>[2x]MRPETIPGISLNEDNSHYFYTRAGRRLSAEEVDSWVDQYAGTQVKELMLCPNCMRTSYASQVWDPIWRGYDPAGPDDQPLLASLPPEERVAARGWIHTAWQLHQDGIDIYARWIRRCRQRGISPWISMRMNDVHYVNDERCFLHSEFWRENPQLRRVPYRFAEWTDRAFDYGRAEVREHH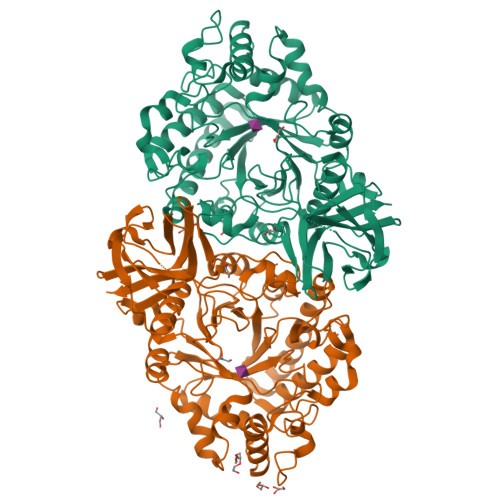LKLIRELAARYDFDGLELDWMRFGFHFRPGYEAEGAEILTAFTAEVRRLLDDWEKRRGHKIHLGARIPSRPATALGLGMDAVTWARRGLVDMLVITPFWASAETDMPVEIWRQLLEGTGVTLAAGLEVLLRPYPDSPLFQTNSLETVRGAAASLLDRGAQRIYLFNYMDSQTAMEDLENYPTLLREIGSLETLAGKPRRHVLTFADTWAPGEPRAIPLPATCRPGEWRAFRLHTGPKPEPGEVIAALGIEGGVAIGPETLEVRVNGELCAFLGLVDLSKPRPDFPVYGFSVPLAAMRRGYNLIEVTARQELRFGWAEFLIRPWHSHHHHHH> MAKVRIYQLAKELGMETQELLELLDQMGVAYKSHASTLEEKDAEAVRELVKEQRGLQEKLAEEERRKSLPRRPPVVVIMGHVDHGKTTLLDYLRKSRIAEKEGGGITQHVGAFEVKTPQGTVVFIDTPGHEAFTTIRQRGAKVADIAVIVIAADDGIMPQTEEAIAHAKAAGAKLIFAINKIDLPQADPEKVKRQLMERGFVPEEYGGDAIVIPISAKTGQGVQDLLEMILLLAELEDYRADPNAEPRGVILESKLDKQAGIIANMLVQEGTFRVGDYVVAGEAYGRIRAMMDADGNQRKEAGPGSAVQVLGFQELPHAGDVVEWVPDLEAAKEIAEERKEERKAREEEEKARRPRTMAELLR

Translation initiation factor 2 (IF2) is involved in the early steps of bacterial protein synthesis. It promotes the stabilization of the initiator tRNA on the 30S initiation complex (IC) and triggers GTP hydrolysis upon ribosomal subunit joining. IF2 is also responsible for the fast subunit association and 70S IC formation, an event that is directly coupled to the activation of the IF2 GTPase. Here, we present the crystal structure of the eubacterial IF2 core as the individual apoprotein and in GTP-bound and GDP-bound forms.

The structure of the apoprotein was determined by multi-wavelength anomalous dispersion (MAD) phasing using selenomethionine and was refined to 1.95 Å resolution. The G domain contains two rather flexible loops (switch I and II; residues 97–103 and 130–139, respectively) which adopt different conformations in the apo, GTP-bound and GDP-bound states. The switch I conformation varies significantly between the apo and nucleotide-bound states, probably owing to the presence of two glycines (RIAEK­EAGG sequence) which are highly conserved and provide flexibility (as also illustrated by higher B factors). In the apo state the side chain of His130 is not visible in the map, indicating that its role is nucleotide-dependent.> QDTSPDTLVVTANRFEQPRSTVLAPTTVVTRQDIDRWQSTSVNDVLRRLPGVDITQNGGSGQLSSIFIRGTNASHVLVLIDGVRLNLAGVSGSADLSQFPIALVQRVEYIRGPRSAVYGSDAIGGVVNIITTRDEPGTEISAGWGSNSYQNYDVSTQQQLGDKTRVTLLGDYAHTHGYDVVAYGNTGTQAQTDNDGFLSKTLYGALEHNFTDAWSGFVRGYGYDNRTNYDAYYSPGSPLLDTRKLYSQSWDAGLRYNGELIKSQLITSYSHSKDYNYDPH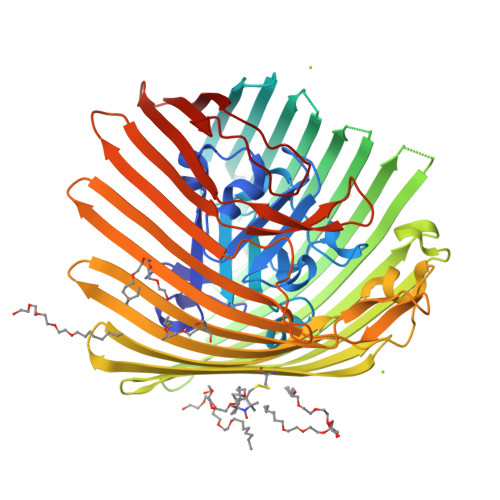YGRYDSSATLDEMKQYTVQWANNVIVGHGSIGAGVDWQKQTTTPGTGYVEDGYDQRNTGIYLTGLQQVGDFTFEGAARSDDNSQFGRHGTCQTSAGWEFIEGYRFIASYGTSYKAPNLGQLYGFYGNPNLDPEKSKQWEGAFEGLTAGVNWRISGYRNDVSDLIDYDDHTLKYYNEGKARIKGVEATANFDTGPLTHTVSYDYVDARNAITDTPLLRRAKQQVKYQLDWQLYDFDWGITYQYLGTRYDKDYSSYPYQTVKMGGVSLWDLAVAYPVTSHLTVRGKIANLFDKDYETVYGYQTAGREYTLSGSYTF> MATILLSAAGAAIGGGFGGTVLGLSGAVIGRAVGATLGRVIDQRLLGSGSQSVETGRVDRLRLSSASEGEAVGRLWGRMRVAGQVIWATRFFESASVEKSGKGVPRATVTSYSYSLSLALALCEGEILRVGRVWADGSEIEVSGLNMRVYRGGEDQLPDPKIAAVEGAEAAPAYRGIAYVVLEDLQLAPFGNRVPQFTFEVVRAAQGALAEAEPDLTRGLRAVALIPGTGEYALATTPVYLATGSGVTATQGVANQNAPGGQTDLVAALERLDEELPNCGAVSLVVSWFGDDLRCGACDVKPKVASVAEEGANMPWRVAGLERAGAEEVPRLSGQSVYGGTPADAAVIEAIAALRAAGKAVTFYPFILMAQLAGNGLPDPWNPGSAQPALPWRGRITLSVAPGRAGSPDGTAAAEAQVAGFFGAASPGDSAIAGGEVVYSGPEEWSMRRFILHYAHLCQLAGGVDAFCIGTEMVALTQIRGPSNSFPAVAAFRQLAGEVKAILGPGCKIGYAADWSEYWGYAPGNGERFFHLDPLWADENIDFIGIDNYLPL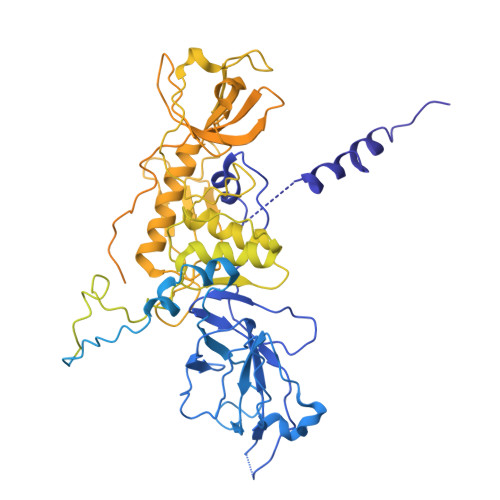SDWRDGADHADAGWGSIHALDYLRSNIEGGEYYDWFYAAPEHRAAQIRTPITDGDHDEPWIWRAKDLRNWWLNDHHERVGGLRSEVATAWVPQSKPIWFTEMGCAAIDKGTNQPNKFLDPKSSESGLPHHSDGRRDELIQMQYLRAMTGYWGEAARNPVSAVYGGPMLDMSRAHVWAWDARPWPQFPLNTALWSDGENYARGHWISGRAVAQPLASVVAEICGAAGITEIDVSGLYGLVRGYTMTGDQTGRAGLQALMLAYGFEALERDGQLVFRMRDGRVAADLAAADLALGEGEAVVETVRAAEAEIAGRVRLAYVEAEGDFEVKAVEAVFPDAAAGAAAGSELSLALTRAQAQGIVGRWLAEARVARDTARFALPPSRGHLGTGDVVRLDLPEGKRRYRIDRVEQAGLIQVEAVRVEPGIYAPADEVEDPASLRPFAAPVPVTAVFLDLPLMKGDEDPVAPHLAVTATPWPGTVAVWSSDEDAGYALNASLGTRAVIGQTLTPLFRARPGVWDRGAALRVRLASGALDSATAAKVLNGANAMAIGDGSSENWEVFQFAEAALVEGKIWDISLRLRGQLGTDALMPEVWPEGSVVVALNGAPEQILLPSAARGLARHYRIGAAVRSYDDPSFVHRIEAFAGAGLRPFSPCHLRAEPGASGWAFRWVRRTRIDGDSWQGYEVPLGETAELYLVRVLEGTAVKREVTVGEASWSYPAALQAADGIAGAFTLEVAQVSDVYGPGLAARITVGA>[2x]MGSSHHHHHHSSGMISNRFGQFIDNELADSMISAEKVAHVQLGNNLEHAL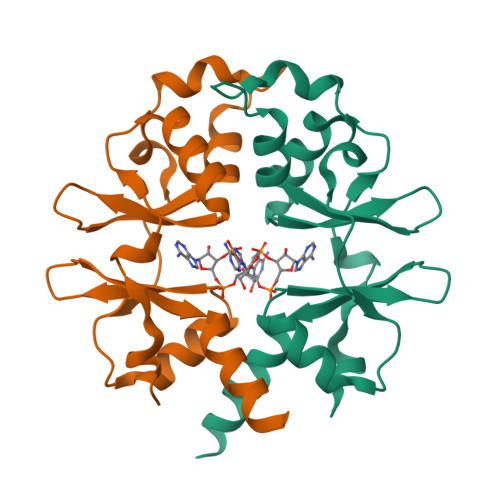LVLTKCGYSVIPVLDFEFKLHGLISAAMITDAILGLERIEFERLEDLKVEDVMQTDFPVIKDFNNNERIVHLLVDHPFVCVVDSDHHFEGIVTRRVVLKQVNRYIHLQVEENR> HHHHHHENLYFQSSEKEELFEKLKQTADEAVQLFQRLREIFDKGDDDSFEQVLEELEEALQKHRQLADQGRKKGLLTSEAAKQGDQFVQLFQRFR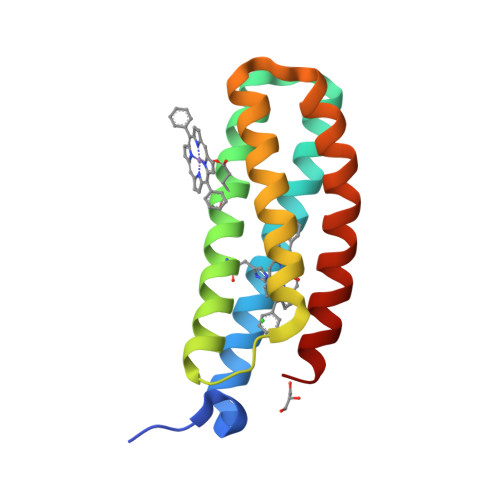EAWDKGDKDSLEQILEELEQVAQKAVELGLKILKTQ> G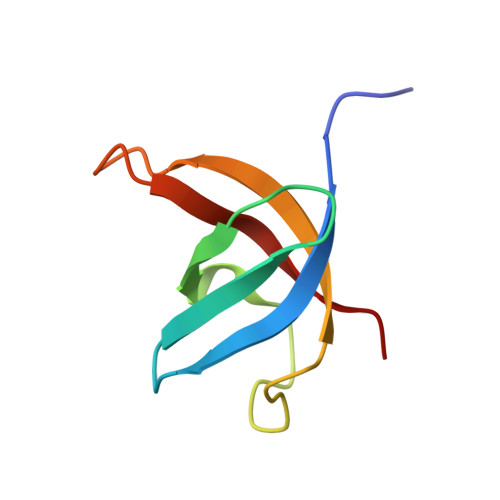AMATRETGIIEKLLHSYGFIQCCERQARLFFHFSQFSGNIDHLKIGDPVEFEMTYDRRTGKPIASQVSKIA> MIFSVDKVRADFPVLSREVNGLPLAYLDSAASAQKPSQVIDAEAEFYRHGYAAVHRGIHTLSAQATEKMENVRKRASLFINARSAEELVFVRGTTEGINLVANSWGNSNVRAGDNIIISQMEHHANIVPWQMLCARVGAELRVIPLNPDGTLQLETLPTLFDEKTRLLAITHVSNVLGTENPLAEMITLAHQHGAKVLVDGAQAVMHHPVDVQALDCDFYVFSGHKLYGPTGIGILYVKEALLQEMPPWEGGGSMIATVSLSEGTTWTKAPWRFEAGTPNTGGIIGLGAALEYVSALGLNNIAEYEQNLMHYALSQLESVPDLTLYGPQNRLGVIAFNL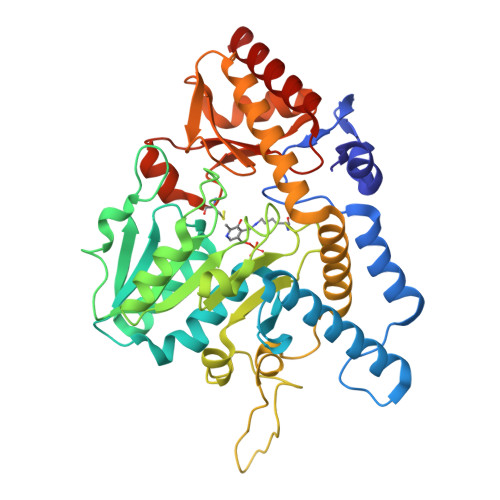GKHHAYDVGSFLDNYGIAVRTGHHCAMPLMAYYNVPAMCRASLAMYNTHEEVDRLVTGLQRIHRLLG> MSLRIDPLGGESLKNQEVKGKKSGKTSRVGESKKKEFFDILEDVKED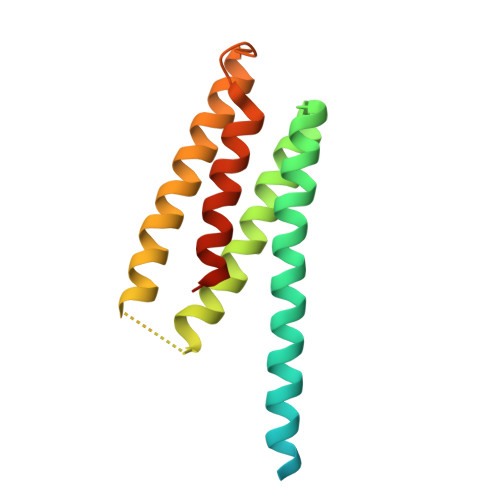HFEKLLEEAVEEVIDSGNELVRSPTPSNLKRYKNAIKEFLKLIEKKIYKLAGSFDMNSGRARLHLVVEEVNEKLMDLTEKIMKNEWQTINLAARIEEINGLILNLYREGHHHHHH> DIIDVNGITIDKNAFKVTVNGAEIELTKTEYDLLYLLAENKNHVMQREQILNHVWGYNSEVETNVVDVYIRYLRNKLKPYDRDKM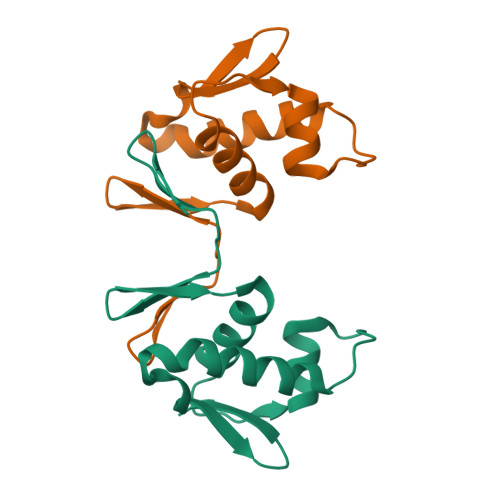IETVRGVGYVIR> MRMFRITACVPSQTRIRTQRELQ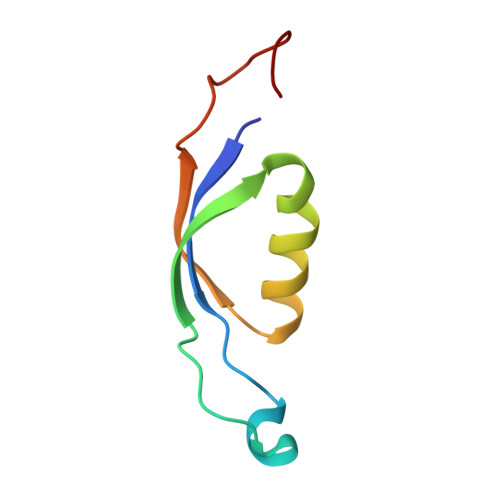NTYFTKLVPYDNWFREQQRIMKMGGKIVKVELATGRPGTNAGLA>[3x]MAHHHHHHHRSPTRVNDGVDADEVTFVNRFTVHGAPAEFES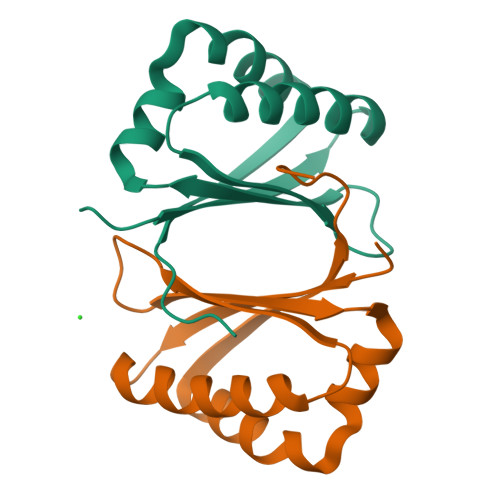VFARTAAFFARQPGFVRHTLLRERDKDNSYVAIAVWTDHDAFRRALAQPGFLPHATALRALSTSEHGLFTARQTLPEGGDTTGSGHR> MGQALGIKSCDFQAARNNEEHHTKALSSRRLFVRRGQPFTIILYFRAPVRAFLPALKKVALTAQTGEQPSKINRTQATFPISSLGDRKWWSAVVEERDAQSWTISVTTPADAVIGHYSLLLQVSGRKQLLLGQFTLLFNPWNREDAVFLKNEAQRMEYLLNQNGLIYLGTADCIQAESWDFGQFEGDVIDLSLRLLSKDKQVEKWSQPVHVARVLGALLHFLKEQRVLPTPQTQATQEGALLNKRRGSVPILRQWLTGRGRPVYDGQAWVLAAVACTVLRCLGIPARVVTTFASAQGTGGRLLIDEYYNEEGLQNGEGQRGRIWIFQTSTECWMTRPALPQGYDGWQILHPSAPNGGGVLGSCDLVPVRAVKEGTLGLTPAVSDLFAAINASCVVWKCCEDGTLELTDSNTKYVGNNISTK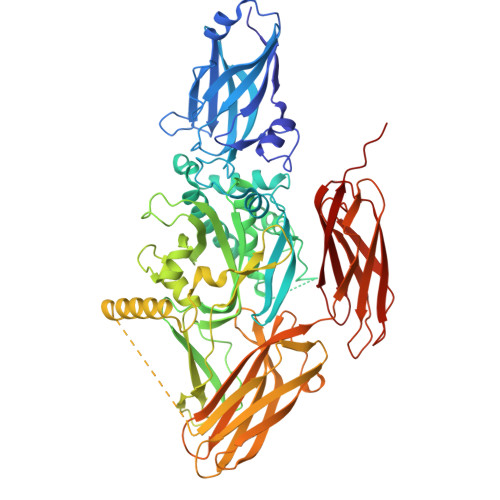GVGSDRCEDITQNYKYPEGSLQEKEVLERVEKEKMEREKDNGIRPPSLETASPLYLLLKAPSSLPLRGDAQISVTLVNHSEQEKAVQLAIGVQAVHYNGVLAAKLWRKKLHLTLSANLEKIITIGLFFSNFERNPPENTFLRLTAMATHSESNLSCFAQEDIAICRPHLAIKMPEKAEQYQPLTASVSLQNSLDAPMEDCVISILGRGLIHRERSYRFRSVWPENTMCAKFQFTPTHVGLQRLTVEVDCNMFQNLTNYKSVTVVAPELSA> GAMASSKLNEDISLIEKQTSGRIGVSVWDTQTDERWDYRGDERFPLMSTFKTLACATMLSDMDSGKLNKNATARIDERNIVVWSPVMDKLAGQSTRIEHACEAAMLMSDNTAANLVLNEIGGPKAVTLFLRSIGDKATRLDRLEPHLNEAKPGDKRDTTTPNAMVNTLHTLMEDNALSYESRTQLKIWMQDNKVSDSLIRSVLPKGWSIADRSGAGNYGSRGISAMIWKDNYKPVYISIYVTD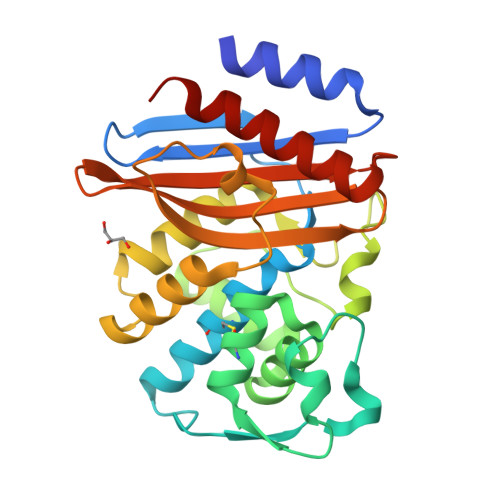TDLSLQARDQLIAQISQLILEHYKES2-(4-ethoxyphenyl)ethanoic acid | C10 H12 O3 | 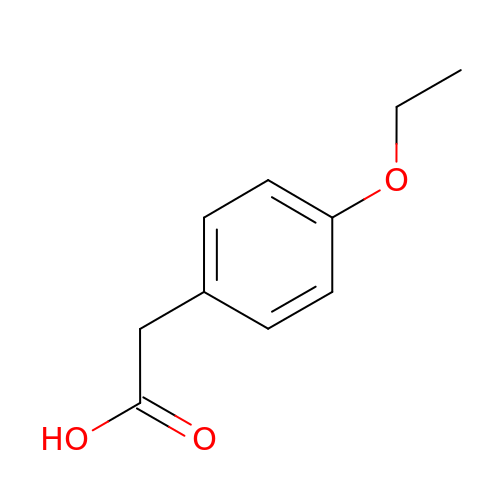ZVVWZNFSMIFGEP-UHFFFAOYSA-N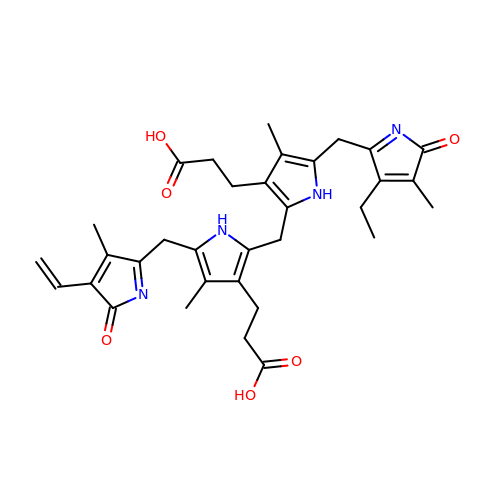3-[5-[(4-ethenyl-3-methyl-5-oxidanylidene-pyrrol-2-yl)methyl]-2-[[5-[(3-ethyl-4-methyl-5-oxidanylidene-pyrrol-2-yl)methyl]-3-(3-hydroxy-3-oxopropyl)-4-methyl-1~{H}-pyrrol-2-yl]methyl]-4-methyl-1~{H}-pyrrol-3-yl]propanoic acid | C33 H38 N4 O6 | UETWWFBMDBJSDH-UHFFFAOYSA-N>[4x]SADVAGAVIDGAGLGFDVLKTVLEALGNVKRKIAVGIDNESGKTWTAMNTYFRSGTSDIVLPHKVAHGKALLYNGQKNRGPVATGVVGVIAYSMSDG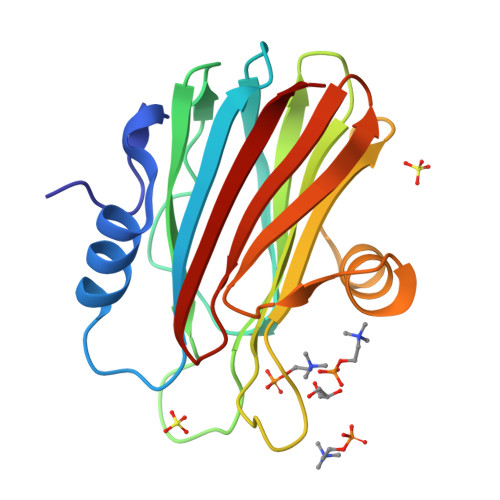NTLAVLFSVPYDYNWYSNWWNVRVYKGQKRADQRMYEELYYHRSPFRGDNGWHSRGLGYGLKSRGFMNSSGHAILEIHVTKA> GQQPVNHLVKEIDMLLKEYLLSGDISEAEHCLKELEVPHFHHELVYEAIVMVLESTGESAFKMILDLLKSLWKSSTITIDQMKRGYERIYNEIPDINLDVPHSYSVLERFVEECFQAGIISKQ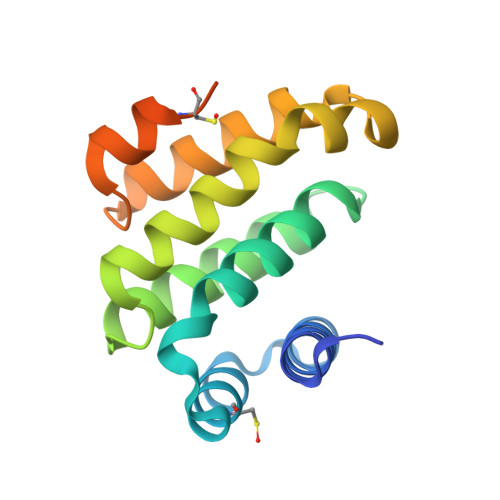LRDLCPSRGRKRFVSEGDGGRLKPESY>MAAPGSRLEPPPLPEYSCSYVVSRPVYSELAFQQQYERRLQERKTLRESLAKRCSCSRKRTLGVLKTLLPVLDWLPKYRIKEWLLSDIISGVSTGLVGTLQGMAYALLAAVPVGYGLYSAFFPILTYFIFGTSRHISVGPFPVVSLMVGSVVLSMAPDEHFIISSSNGTALNTTVIDFAARDAARVLIASTLTLLVGIIQLIFGGLQIGFIVRYLADPLVGGFTTAAAFQVLVSQLKIVLNVSTKNYNGILSIIYTLIEIFQNIGNTNLADFIAGLLTIIICMAVKELNDRFKHKIPVPIPIEVIVTIIATAISYAVNLEKNYNAGIVKSIPRGFLPPEIPPISLFSEMLTASFSIAVVAYAIAVSVGKVYAIKYDYTIDGNQEFIAFGISNIFSGFFSCFVATTALSRTAVQESTGGKTQIAGIISAAVVMIAIVALGKLLEPLQKSVLAAVVIANLKGMFMQVCDVPRLWRQNKTDAVIWVFTCIASIILGLDLGLLAGLMFGFLTVVVRVQFPSWNSLGSIPNTDIYRSTKDYKNIEEPEGVKILRFSSPIFYGNVDGLKKCIKSTVGFDAIRVYNKRLKALRKIQKLIKKGQLRATKNGIISDAGSSNNAFEPDEDIEDPEELDIPTKEIEIQVDWNSELPVKVNVPKVPIHSLVLDCGAVSFLDVVGVRSLRMIVKEFQRIDVHVYFASLQDHVIEKLEQCGFFNDSIRKDIFFLTVHDAILHLRSQVKSQEVQDSILETITLIQDCKDPLELMEAELIEEELDVQDEAMRRLAS[2x]

Pendrin (SLC26A4) is an anion exchanger that mediates bicarbonate (HCO3−) exchange for chloride (Cl−) and is crucial for maintaining pH and salt homeostasis in the kidney, lung, and cochlea. Pendrin also exports iodide (I−) in the thyroid gland. Pendrin mutations in humans lead to Pendred syndrome, causing hearing loss and goiter. Here, we present structures of pendrin from Sus scrofa (ssPendrin), which is 90% identical to human pendrin, in complex with either I−, HCO3−, or Cl−; ssPendrin in the apo-state; and ssPendrin in the presence of NFA, which inhibits anion transport.

The structures of ssPendrin in the presence of I−, HCO3− or Cl− were determined by cryo-electron microscopy (cryo-EM) to an overall resolution of 2.8 Å, 2.7 Å, and 2.5 Å, respectively. Since the three structures have only minor differences, we describe the Cl−-bound ssPendrin here. The final structural model includes residues 17 to 39, 64 to 585, and 654 to 732, which resolves all 14 transmembrane helices and their connecting loops and most of the STAS domain. TM3 and TM10 cross roughly in the center of the membrane, and together with residues from TM1 and TM8, form a cradle for substrate anions. The anion in S1 is coordinated by the backbone hydrogens of Leu407 and Ser408 and the side chain hydroxyl hydrogen of Ser408. The side of the aromatic ring of Phe141 from TM3 is within 4.0 Å of S1 and could stabilize the anion in S1 by anion-π interactions. The anion at the S2 position is coordinated by the sidechain hydroxyl hydrogen of Tyr105 and sidechain amide hydrogens of Gln101 and Asn457. While the anion in S1 is coordinated within the transport domain, the anion of S2 involves residue Asn457, which is on TM12 from the scaffold domain. In all three ssPendrin structures, the anion binding sites are solvent accessible from the intracellular side through a large cavity formed between the transport and scaffold domains. Thus, the structures of ssPendrin are captured in the inward-facing conformation.> ELTPDQQTLLHFIMDSYNKQRMPQEITNKILKEEFSAEENFLILTEMATNHVQVLVEFTKKLPGFQTLDHEDQIALLKGSAVEAMF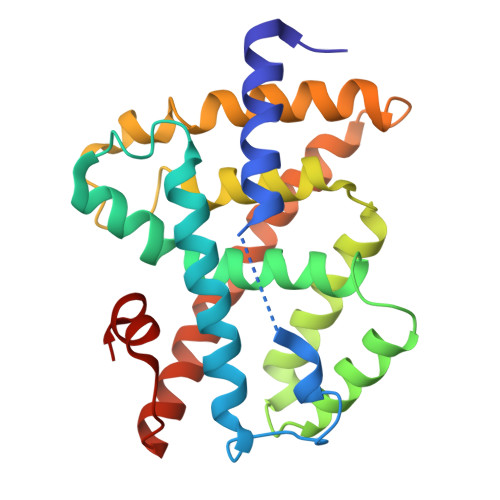LRSAEIFNKKLPSGHSDLLEERIRNSGISDEYITPMFSFYKSIGELKMTQEEYALLTAIVILSPDRQYIKDREAVEKLQEPLLDVLQKLCKIHQPENPQHFACLLGRLTELRTFNHHHAEMLMSWRVNDHKFTPLLCEIWDVQ>AECSVDIQGNDQMQFNTNAITVDKSCKQFTVNLSHPGNLPKNVMGHNWVLSTAADMQGVVT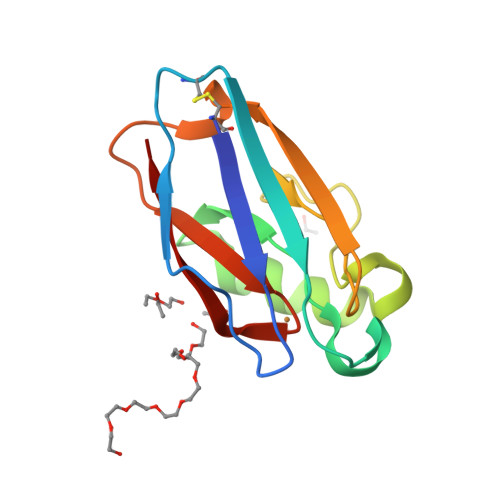DGMASGLDKDYLKPDDSRVIAHTKLIGSGEKDSVTFDVSKLKEGEQYMFFCTPHPFMKGTLTLK[4x]> MALSDLQVFNDWAYKTMSEVLDQQVELFNGATRGAIILRSAGNTGDLSEAAFWAKIQGLVRPRDPYSNADVAAKDLRQLVDNTIKVASGTPPINIPPSMLRWIQKNPQEAGAVIGQQLAGDTMQDMLNNGLAAGKAAFTAGGAVHDISAAGTGLMTQRAFNAAQRIFGDRSTDIQVWVSHSSP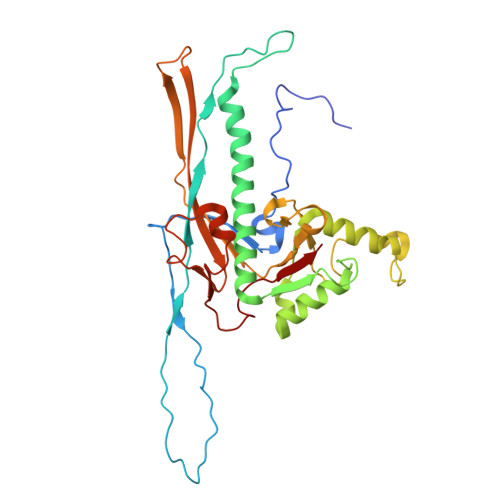LFDLYDNALANAEQLYVFGTVNVRADAFGRPIIITDSPALVSGAAETLRHSTLGLTTGAILIEQNQDFDSTVVDGTGKQNITRQYQAEWSYNLGVNGYAYDIATGGKAPNPTALATAANWDKISTSIKDTGGVVLVTK> RYILPSFIEHSSFGVKESNPYNKLFEERIIFLGVQVDDASANDIMAQLLVLESLDPDRDITMYINSPGGGFTSLMAIYDTMQYVRADIQTVCLGQAASAAAVLLAAGTPGKRMALPNARVLIHQPSLSGVIQGQFSDLEIQAAEIERMRTLMETTLARHTGKDAGVIRKDTDRDKILTAEEAKDYGIIDTVLEYRKLSAQ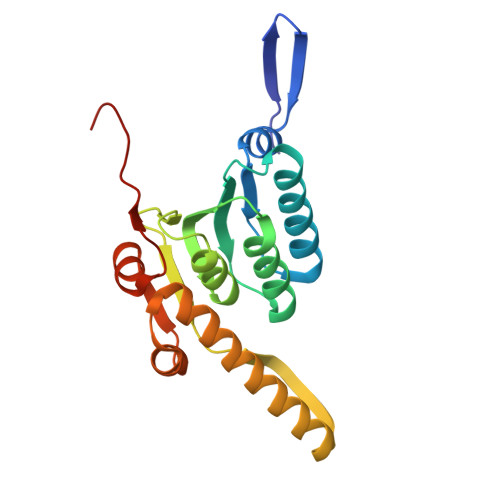TA>[3x]GPGSMEASCLELALEGERLCKSGDCRAGVSFFEAAVQV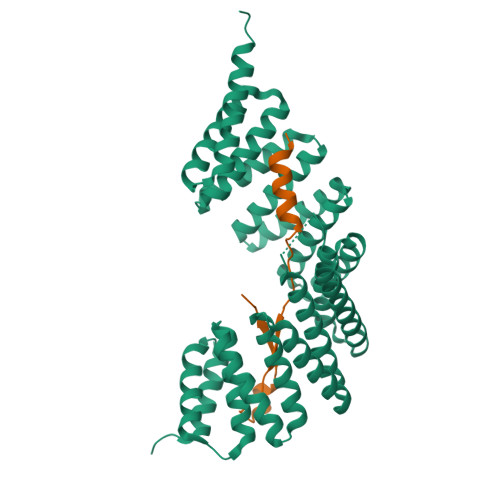GTEDLKTLSAIYSQLGNAYFYLHDYAKALEYHHHDLTLARTIGDQLGEAKASGNLGNTLKVLGNFDEAIVCCQRHLDISRELNDKVGEARALYNLGNVYHAKGKSFGCPGPQDVGEFPEEVRDALQAAVDFYEENLSLVTALGDRAAQGRAFGNLGNTHYLLGNFRDAVIAHEQRLLIAKEFGDKAAERRAYSNLGNAYIFLGEFETASEYYKKTLLLARQLKDRAVEAQSCYSLGNTYTLLQDYEKAIDYHLKHLAIAQELNDRIGEGRACWSLGNAYTALGNHDQAMHFAEKHLEISREVGDKSGELTARLNLSDLQMVLGLSYSTNNSIMSENTEIDSSLNGVRPKLGRRHSMENMELMKLTPEK;>[3x]GPLGSMQVDSVQRWMEDLKLMTECECMCVLQAKPISLEEDAQGDLILAGGPG>[2x]ETGYGPEDVLKFVGNESVVDHFKLVTKDGNSLLIGARNTVFNLSIHDLVEQQRLVWTSPEDDTKMCLVKGKDEEACQNYIRIMVVPSPGRLFVCGTNSFRPMCNTYIISDSNYTLEATKNGQAVCPYDPRHNSTSVLADNELYSGTVADFSGSDPIIYREPLQTEQYDSLSLNAPNFVSSFTQGDFVYFFFRETAVEFINCGKAIYSRVARVCKWDKGGPHRFRNRWTSFLKSRLNCSIPGDYPFYFNEIQSASNLVEGQYGSMSSKLIYGVFNTPSNSIPGSAVCAFALQDIADTFEGQFKEQTGINSNWLPVNNAKVPDPRPGSCHNDSRALPDPTLNFIKTHSLMDENVPAFFSQPILVRTSTIYRFTQIAVDAQIKTPGGKTYDVIFVGTDHGKIIKSVNAESADSADKVTSVVIEEIDVLTK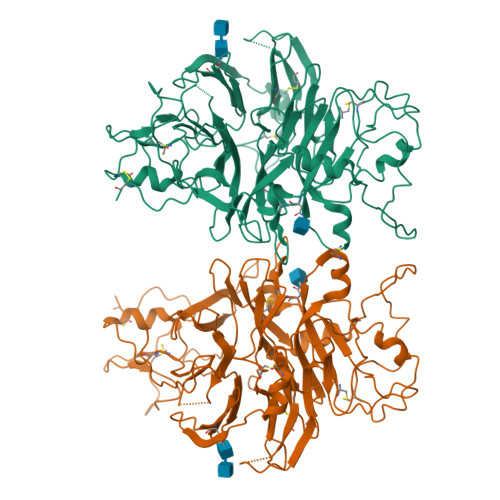SEPIRNLEIVRTMQYDQPKDGSYDDGKLIIVTDSQVVAIQLHRCHNDKITSCSECVALQDPYCAWDKIAGKCRSHGAPRWLEENYFYQNVATGQHAACPSGTKHHHHHH>[2x]MRVGVLGAKGKVGTTMVRAVAAADDLTLSAELDAGDPLSLLTDGNTEVVIDFTHPDVVMGNLEFLIDNGIHAVVGTTGFTAERFQQVESWLVAKPNTSVLIA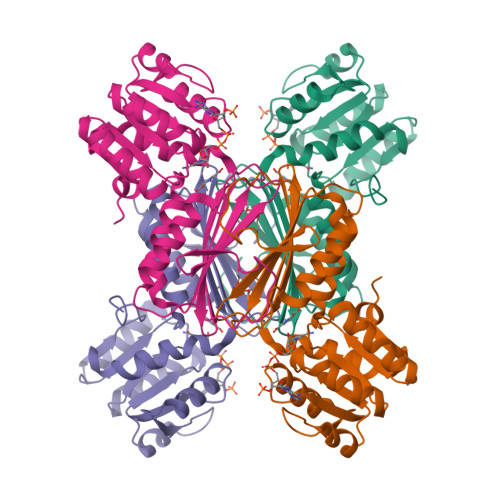PNFAIGAVLSMHFAKQAARFFDSAEVIELHHPHKADAPSGTAARTAKLIAEARKGLPPNPDATSTSLPGARGADVDGIPVHAVRLAGLVAHQEVLFGTEGETLTIRHDSLDRTSFVPGVLLAVRRIAERPGLTVGLEPLLDLH Prolonged signalling, particularly by inflammatory cytokines, is detrimental to both the cell and the organism, and is therefore tightly regulated, in particular, by the SOCS (Suppressors of Cytokine Signalling) family of proteins. We have determined its mode-of-action by solving two X-ray crystal structures of SOCS1 bound to its physiological targets (both the ElonginB/C adapter complex and also the JAK1 kinase domain). SOCS1 is shown to be a direct inhibitor of the catalytic activity of JAK1, JAK2 and TYK2 but not JAK3. Our structure reveals that SOCS1 inhibits these three JAK family members by blocking the substrate binding groove on JAK, acting as a pseudosubstrate.

To structurally characterise the mechanism of SOCS1 inhibition of JAK kinase activity, we solved the structure of Gallus gallus SOCS1, without its SOCS Box domain, in complex with the human JAK1 kinase domain bound to ADP, using X-ray crystallography (ggSOCS1ΔSOCSbox-JAK1KD). Attempts to crystallise a complex containing human SOCS1 were unsuccessful, however, the Gallus gallus and human orthologues share 72% identity and 89% similarity and display similar efficacy in JAK inhibition, indicating that it is a good model for the human protein. Crystals of a 1:1 complex were obtained and the data processed to 2.5 Å. SOCS1 binds to JAK using both its SH2 domain and kinase inhibitory region. The interface between the two proteins is 1159 Å2 and the KIR of SOCS1 is responsible for approximately half of this buried surface. The significantly improved resolution of the SOCS1/JAK1 structure allows a detailed atomic-level analysis of this interaction and shows that it is mediated by a continuous six residue segment of the KIR (His54 to Arg59), corresponding to residues −1 to +5 of this motif based on earlier definitions. The first of these, His54, is sandwiched between two planar sidechains from JAK1, the upper sidechain is from His885 in the glycine-rich loop of the kinase and the lower sidechain is Pro1044. Phe55 is the P + 1 mimicking residue and, together with Phe58, form the bulk of the hydrophobic interactions (with Phe1046, Thr1100 and Val1101 from JAK1) that wedge the KIR between the activation loop and the αG helix as well as providing three mainchain-derived hydrogen bonds. When bound to SOCS1, the JAK1 kinase domain adopts an active conformation, characterised by the activation loop displaced from the ATP-binding site with a DFG-in position, an intact substrate-binding groove and both the C-spine and R-spine26 aligned. The activation loop is in its active conformation and this is notable because Tyr1034 is unphosphorylated.

> AHFEKRFLKRIRDLGEGHFGKVELCRYDPEGDNTGEQVAVKSLKPESGGNHIADLKKEIEILRNLYHENIVKYKGICTEDGGNGIKLIMEFLPSGSLKEYLPKNKNKINLKQQLKYAVQICKGMDYLGSRQYVHRDLAARNVLVESEHQVKIGDFGLTKAIETDKEYYTVKDDRDSPVFWYAPECLMQSKFYIASDVWSFGVTLHELLTYCDSDSSPMALFLKMIGPTHGQMTVTRLVNTLKEGKRLPCPPNCPDEVYQLMRKCWEFQPSNRTSFQNLIEGFEALL;> STHFRTFRSQADFSSITRASSLLDACGFYWGPLTVSAAHEKLKSEPEGTFLIRDSTQKNCFFAISVKTATGPTSIRINFQTGRFSLDGSKETFDCLFKLLEHYLSSPRKVLVTPLRK> MNNLYRDLAPITESAWAEIELEATRTFKRHIAGRRVVDVSGPNGPT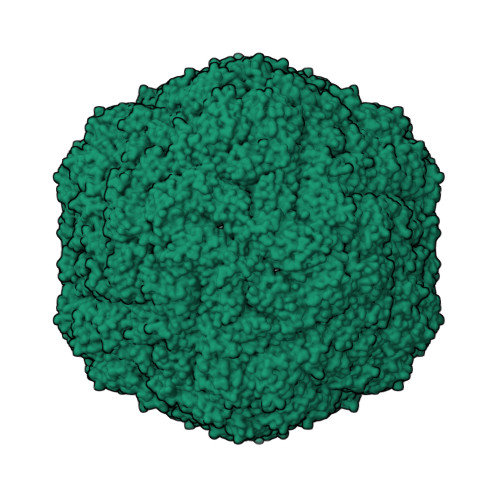TASVSTGHLLDVSPPGDGVIAHLRDAKPLVRLRVPFTVARRDIDDVERGSQDSDWDPVKDAAKKLAFVEDRAIFEGYAAASIEGIRSSSSNPALALPDDAREIPDVIAQALSELRLAGVDGPYSVLLSAETYTKVSETTAHGYPIREHINRLVDGEIIWAPAIDGAFVLSTRGGDFDLQLGTDVSIGYLSHDAEVVHLYMEETMTFLCYTAEASVALTP> MGNRGMEDLIPLVNRLQDAFSAIGQNADLDLPQIAVVGGQSAGKSSVLENFVGRDFLPRGSGIVTRRPLVLQLVNATTEYAEFLHCKGKKFTDFEEVRLEIEAETDRVTGTNKGISPVPINLRVYSPHVLNLTLVDLPGMTKVPVGDQPPDIEFQIRDMLMQFVTKENCLILAVSPANSDLANSDALKVAKEVDPQGQRTIGVITKLDLMDEGTDARDVLENKLLPLRRGYIGVVNRSQKDIDGKKDITAALAAERKFFLSHPSYRHLADRMGTPYLQKVLNQQLTNHIRDTLPGLRNKLQSQLLSIEKEVEE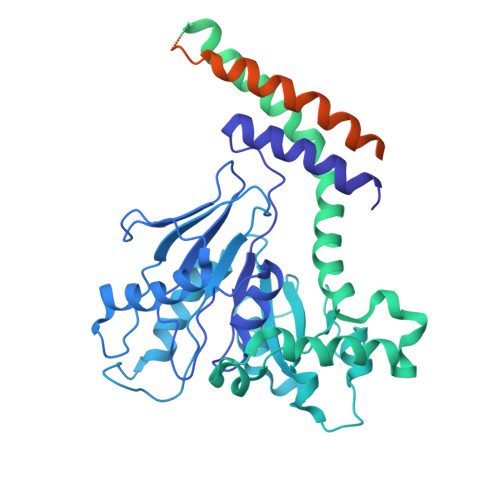YKNFRPDDPARKTKALLQMVQQFAVDFEKRIEGSGDQIDTYELSGGARINRIFHERFPFELVKMEFDEKELRREISYAIKNIHGIRTGLFTPDMAFETIVKKQVKKIREPCLKCVDMVISELISTVRQCTKKLQQYPRLREEMERIVTTHIREREGRTKEQVMLLIDIELAYMNTNHEDFIGFANAQQRSNQMNKKKTSGNQDEILVIRKGWLTINNIGIMKGGSKEYWFVLTAENLSWYKDDEEKEKKYMLSVDNLKLRDVEKGFMSSKHIFALFNTEQRNVYKDYRQLELACETQEEVDSWKASFLRAGVYPERVGDKEKASETEENGSDSFMHSMDPQLERQVETIRNLVDSYMAIVNKTVRDLMPKTIMHLMINNTKEFIFSELLANLYSCGDQNTLMEESAEQAQRRDEMLRMYHALKEALSIIGNINTTTVSTPMPPPVDDSWLQVQSVPAGRRSPTSSPTPQRRAPAVPPARPGSRGPAPGPPPAGSALGGAPPVPSRPGASPDPFGPPPQVPSRPNRAPPGVPSRSGQASPSRPESPRPPFDL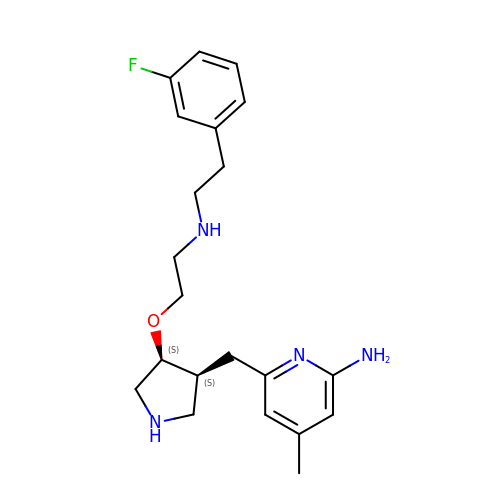6-{[(3S,4S)-4-(2-{[2-(3-fluorophenyl)ethyl]amino}ethoxy)pyrrolidin-3-yl]methyl}-4-methylpyridin-2-amine | C21 H29 F N4 O | NESZTSPBRDBHCW-FXAWDEMLSA-N2-[(3-fluorobenzyl)amino]ethanesulfonic 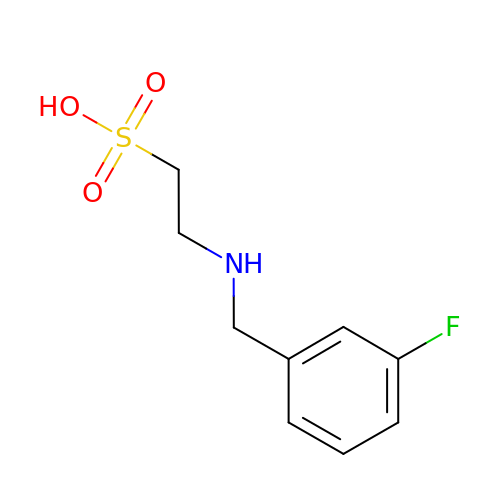acid | C9 H12 F N O3 S | YAVXRLCPJYFRHJ-UHFFFAOYSA-N>[2x]GSNRDPRDHYDLLQRLGGGTYGEVFKARDKVSGDLVALKMVKMEPDDDVSTLQKEILILKTCRHANIVAYHGSYLWLQKLWICMEFCGAGSLQDIYQVTGSLSELQISYVCREVLQGLAYLHSQKKIHRDIKGANILINDAGEVRLAD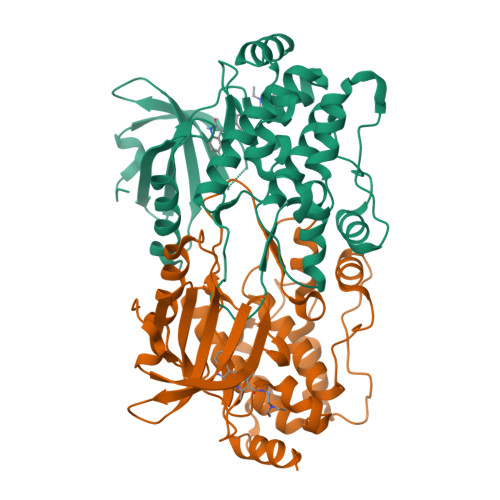FGISAQIGATLARRLSFIGTPYWMAPEVAAVALKGGYNELCDIWSLGITAIELAELQPPLFDVHPLRVLFLMTKSGYQPPRLKEKGKWSAAFHNFIKVTLTKSPKKRPSATKMLSHQLVSQPGLNRGLILDLLDKLKNPGKGPSIGDIEDEE>[2x]MGSYSSDDVEVIREAGRAQGLATILAIGTATPPNCVAQADYADYYFRVTKSEHMVDLKEKFKRICEKTAIKKRYLALTEDYLQENPTMCEFMAPSLNARQDLVVTGVPM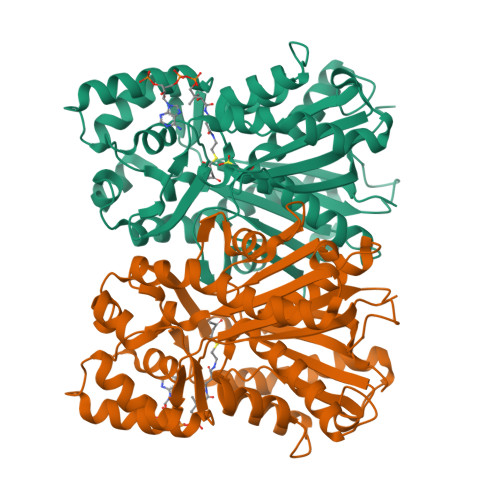LGKEAAVKAIDEWGLPKSKITHLIFCTTAGVDMPGADYQLVKLLGLSPSVKRYMLYQQGCAAGGTVLRLAKDLAENNKGSRVLIVCSEITAILFHGPNENHLDSLVAQALFGDGAAALIVGSGPHLAVERPIFEIVSTDQTILPDTEKAMKLHLREGGLTFQLHRDVPLMVAKNIENAAEKALSPLGITDWNSVFWMVHPGGRAILDQVERKLNLKEDKLRASRHVLSEYGNLISACVLFIIDEVRKRSMAEGKSTTGEGLDCGVLFGFGPGMTVETVVLRSVRVTAAVANGN> AN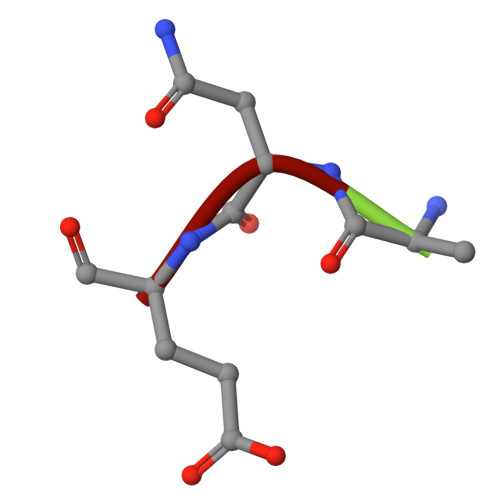E>[2x]GSHMITVATAECFTHANIGLTIHKAAAGYE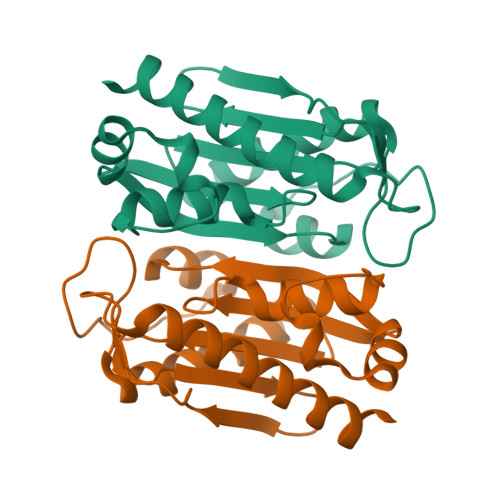DFEFKYLFSEEDLKLMKNVRVISAMFVPSIIGVEKLLDIKLPEPDFNYKYAKAYSEEKDLEVAKLMAEGLKKKLNVNISIGSTAGVGRGAICILTDNNRYLFTSDVYANLITFENIKERQKNGIEKGIKRFLEILKKEYF> GAMDPEFNTWSSSSVEFLDDADDNRLLFTCTFTLPHGTVLSSATYADGFHEQYLTIGDNFLARLEPKGQSFILSAAAASVKQRIFARVTMPDGALRACELLCEFETDRAKITVLALRSAFSL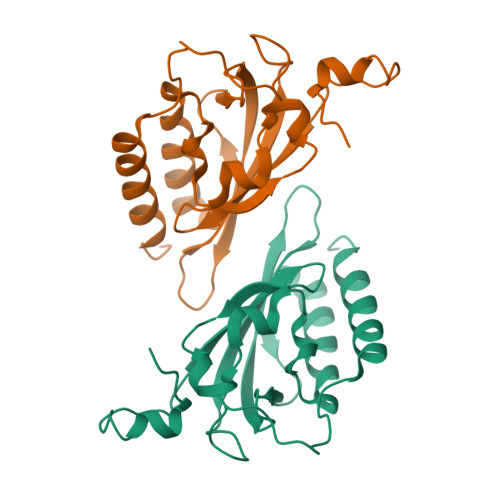QASHVSSNFHVFTFITKHSSTCALTHIDYASIPYLGLLPTDLIGKSLLAFVYSPDVHVVRQAHIDLHNSRGKIVKSIADLRLVAHNGSILRCQTEWSAYVNPWTRKMELVVARHRICSLPIGDSDVISSPPPGIQSNTLPPVMAKTFEDELRTIMNKPVP>GAMATEQIQHIAIVGCVHGKYREMYRQLSEYEKSTGKEISFVICTGDMQTLRYEADLVYLKVPPKYKQMGDFHLYYEGKEKAPYLTLFIGGNHESSNVLLHLYNGGFVCFNMYYLGVCSCININGLRIVGVSGIYKSFDEKKPYTYPPSPNDVVSLFHTRNYVIQMLSNLSQSSQIDISLSHDWPQGIVMKGNYKQLYRFQPGFKKDGASLGSPINKVILNTLKPKYWISGHMHCEYHAEEGPTHFIALGKIGYKNAISYLDLPLKQKTDLEYDKDWVCNLIMTWPAFSNKAQFPDLSYSISELL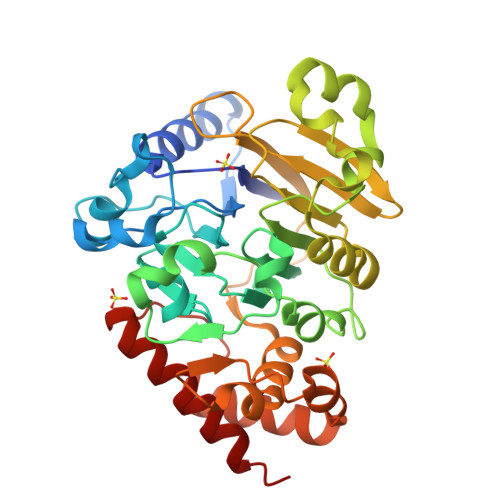SKRTKELDKKIIELWEKYIGLKIIYDSDTFDIQFTSRRFYIEKIYNELNIN[5x]>RQE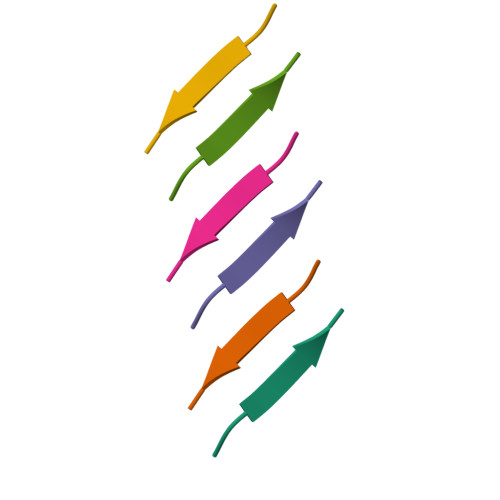FEV[2x]Left-handed G4s are characterized by the anticlockwise rotation of the backbone in its helical progression. They have several unique and distinct structural features, such as: (i) ability to form stable four-layered and bi-layered dimeric structures, (ii) stacking of thymine loops with the outer tetrads (T-capping) and (iii) the local sugar orientation of each base is almost perpendicular to the overall backbone progression giving rise to the ‘twisted’ backbone. Bulges are important structural elements of G4s, which form as protrusions of bases from the G-tetrad core. Here we report on the ability of the 12-nt sequence GTGGTGGTGGTG called LHG4motif to drive several DNA sequences towards left-handed G4s with bulges.

The sequence 2xBulge-LHG4motif-TT with two thymines at the 3′-end was crystallized in the P21 space group with two molecules in the asymmetric unit. The two molecules were related by a translation. The overall structures are noticeably close to each other with an rmsd of 0.112 Å for all non-H superimposed atoms excluding the bulges. Both crystal structures feature four-layered G4s separated into two blocks connected by one thymine linker. In case of 2xBulge-LHG4motif-TT, two thymine residues T5 and T9 are projected outward between guanines G4 and G6 as well as G8 and G10, respectively, in the upper block. The overhang 3′-thymines (TT) stack on the capping thymines. A spermine molecule (from the crystallization solution) stacks over the outer tetrad in each block. The crystal structure of 2xBulge-LHG4motif-TT also displays three potassium ions coordinated in the central channel of the G4. The two molecules (A and B) in the asymmetric unit are closely similar with an rmsd of 0.132 Å for all non-H superimposed atoms. The molecule B was observed to contain one additional potassium ion in close proximity to thymine T22 and one of the spermine molecule. In addition, there is a sodium ion nearby the second bulge T9 in molecule B that interacts with O2 and O4’ of the bulge residue, potentially stabilizing the structure.

>GGTGTGTGTGTGGTGTGGTGGTGGTGTT[2x]> MAHHHHHHMKKLQIAVGIIRNPQGEIFITQRAADAHMANKLEFPGGKIESDETPEQALIRELQEEVGITVTTSSL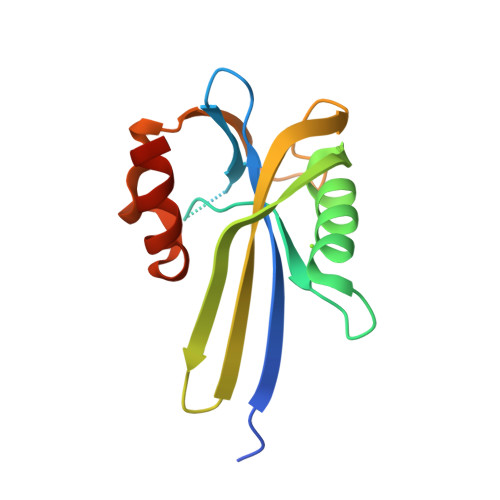FDKLEYQFPDRHITLWFFLVESWQGEPWGKEGQPGRWMAGPTLDPAAFPPANEPVISKLIAQGVSK> TETTSFLITKFSPDQQNLIFQGDGYTTKEKLTLTKAVKNTVGRALYSSPIHIW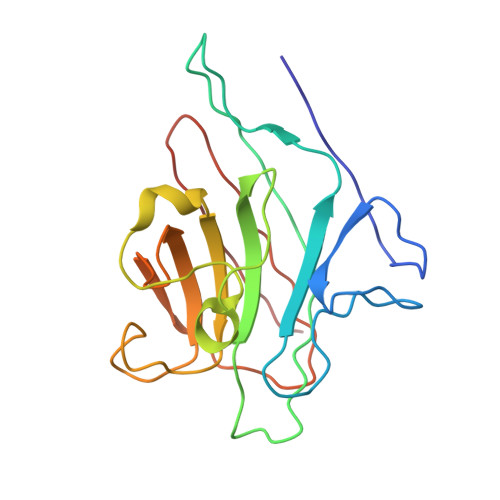DRETGNVANFVTSFTFVINAPNSYNVADGFTFFIAPVDTKPQTGGGYLGVFNSAEYDKTTETVAVEFDTFYNAAWDPSNRDRHIGIDVNSIKSVNTKSWKLQNGEEANVVIAFNAATNVLTVSLTYP>[2x]AAKTEQQIADIVNRTITPLMQEQAIPGMAVAIIYQGKP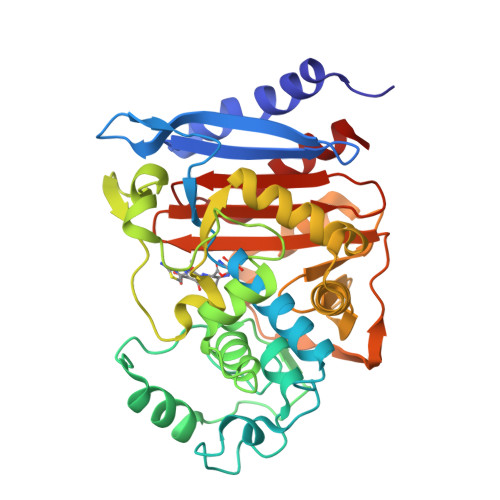YYFTWGKADIANNRPVTQQTLFELGSVSKTFNGVLGGDAIARGEIKLSDPVTQYWPELTGKQWQGISLLHLATYTAGGLPLQVPDDVTDKAALLRFYQNWQPQWAPGAKRLYANSSIGLFGALAVKPSGMSYEEAMSKRVLHPLKLAHTWITVPQSEQKDYAWGYREGKPVHVSPGQLDAEAYGVKSSVIDMTRWVQANMDASQVQEKTLQQGIELAQSRYWRIGDMYQGLGWEMLNWPVKADSIISGSDSKVALAALPAVEVNPPAPAVKASWVHKTGSTGGFGSYVAFVPEKNLGIVMLANKSYPNPVRVEAAWRILEKLQ>MTAPRSWAPTTRARGDTEALCSPEDGWVKVHPTPGTMLFREILHGQLGYTEGQGVYNVVRSSEATTRQLQAAIFHALLNATTYRDLEADWLGHVAARGLQPQRLVRRYRNAREADIAGVAERVFDTWRNTLRTTLLDFAHGLVACFAPGGPSGPSSFPKYIDWLTCLGLVPILRKRQEGGVTQGLRAFLKQHPLTRQLATVAEAAERAGPGFFELALAFDSTRVADYDRVYIYYNHRRGDWLVRDPISGQRGECLVLWPPLWTGDRLVFDSPVQRLFPEIVACHSLREHAHVCRLRNTASVKVLLGRKSDSERGVAGAARVVNKVLGEDDETKAGSAASRLVRLIINMKGMRHVGDINDTVRSYLDEAGGHLIDAPAVDGTLPGFGKGGNSRGSAGQDQGGRAPQLRQAFRTAVVNNINGVLEGYINNLFGTIERLRETNAGLATQLQERDRELRRATAGALERQQRAADLAAESVTGGCGSRPAGADLLRADYDIIDVSKSMDDDTYVANSFQHPYIPSYAQDLERLSRLWEHELVRCFKILCHRNNQGQETSISYSSGAIAAFVAPYFESVLRAPRVGAPITGSDVILGEEELWDAVFKKTRLQTYLTDIAALFVADVQHAALPPPPSPVGADFRPGASPRGRSRSRSPGRTAPGAPDQGGGIGHRDGRRDGRR[10x]

Three capsid types have been recognized from the nuclei of herpesvirus-infected cells: empty A-capsids, scaffolding-containing B-capsids, and DNA-filled C-capsids. A unique portal vertex exists at a 12th I5 vertex through which the genome is translocated during assembly. Here, portal proteins assemble into a dodecameric basket-like structure that is thought to seed the assembly of scaffolding proteins, in turn driving the formation of spherical procapsids composed of MCP, SCP, and triplexes. A separate protein complex, the terminase, associates with the dodecameric portal and initiates genome packaging and the concurrent autoproteolytic cleavage of the scaffold.

The resultant atomic structures reveal not only the expected A-, B-, and C-capsids but also capsids with portal vertices similar to C-capsids but no resolvable genome in the capsid lumen, which we named D-capsids. We refer to these capsids as “D-capsids” because their C-capsid-like portal suggests they were originally C-capsids, but the absence of most of the genome indicates that they are degraded. Ten of the 12 monomers from the basket are linked to the turret helices, each of which consists of one long helix extending toward the portal cap and connecting to two smaller helices arranged in a small helical bundle. The two non-contributing portal monomers are presumably disordered or flexible beginning at their turret sequences. In C-capsids, D-capsids, and virions, the turret helices are fully extended, whereas in A- and B-capsids, they are retracted and positioned ~65 Å lower (Fig. 1F through J).Rai1 homologs share several highly conserved sequence motifs, and our structural studies show that they are located in the active site region, mediating the binding of the divalent metal ions and/or the RNA. We have found substantial variations in the activity profiles of the Rai1 homologs, and discovered that some of them possess a new 5′ triphosphonucleotide hydrolase (TPH) activity. The overall structures of CaRai1, AgRai1 and SsRai1 are similar to those of SpRai1 (16), KlDxo1 (18), and MmDXO. Each structure contains two mixed β-sheets that are surrounded by α-helices.

The CaRai1–pU5–Mn2+ complex was obtained by co-crystallization with pU5 RNA using 1:2 protein:RNA molar ratio in the presence of 10 mM MnCl2. In the CaRai1–pU5–Mn2+ ternary complex, clear electron density was observed for the first four nucleotides of the RNA. Two Mn2+ ions are coordinated by residues in motifs II (Glu174, αD), III (Glu223 and Asp225, β10 and β10–β11 loop) and IV (Glu244, β12), as observed earlier in the MmDXO–pU5–Mn2+ complex. Similarly, one of the terminal oxygen atoms of the 5′ monophosphate, the scissile phosphate of the substrate, is a bridging ligand to both metal ions. Therefore, the RNA is bound as a product of the reaction, and hence its nucleotides are numbered U2 through U5, while nucleotide U1 would be the leaving group of the substrate. The structure revealed that Glu104 (αB) is located near the expected binding site for the 5′ segment of the substrate. The side chain has weak electron density and assumes different conformations in the two CaRai1 molecules in the asymmetric unit. This residue is unique to CaRai1, and is a Gly in the other Rai1 proteins. The presence of the negative charge and the larger size of the side chain could interfere with the binding of the substrate through electrostatic and steric repulsions. The phosphate of U4 has ionic interactions with the side chains of Lys263 (αF, motif V) and Arg284 (β13, motif VI), while that of U5 has ionic interactions with Arg284 (motif VI) and Arg159 (αD). Arg159 is not conserved among Rai1 homologs, and the unique interaction with this residue may have helped define the bound conformation of pU5 to CaRai1.

>[2x]HMAKSLPLNSRSKTTALKQPRELFSYARDIDGKYVYDDPENSLSYYYLPDSTIDTGIDLQGGYSKFKKIPDEQNLADFNSLLKAIIKYETSEGKKISSDIITFREIMTKILSLPYNLTDPIDLYVVPFDGQLFIKSDDELDMKRRKEQEVRMKQTNTVERYDYMKRCEYVGYKFETIATIPKPWSQVSRSQIENRNKKVVNNYEQYLSVIRTGIGNVKLVLAGEIDCCWDYLPDEQNKKLNHYVELKTSRIIENNSQVVSFEQKLFKAWCQCFLMGVTKIIYGFRDNNLILKNVELFNTEEIPILIKNNPLTNAATEKKINCTNALKWYGAVVDWLNTTVDKKDEIKSYRLKYDPVRKSFTLSETDSETNEKLRNGQLLTPEFTEWRQSLKK>[2x]AQEEEAEQNLSELSGPWRTVYIGSTNPEKI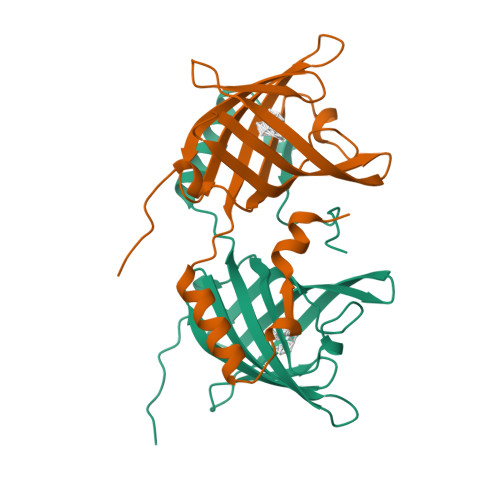QENGPFRTYFRELVFDDEKGTVDFYFSVKRDGKWKNVHVKATKQDDGTYVADYEGQNVFKIVSLSRTHLVAHNINVDKHGQTTELTGLFVKLNVEDEDLEKFWKLTEDKGIDKKNVVNFLENEDHPHPE>NNELSPVALRQMSCAAGTTQTACTDDNALAYYNNSKGGRFVLALLSDHQDLKWARFPKSDGTGTIYTEL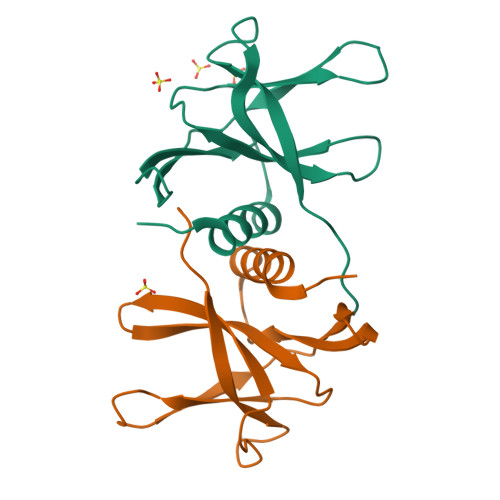EPPCRFVTDTPKGPKVKYLYFIKGLNNLNRGMVLGSLAATVRLQ[2x]> SNATGERFHPLLGRRVLDPAPGARCFTGTVSSDRPAYLGEHWVYDAIVVLGVTYLEMALAAASRLLPGNAADTLIVEDVTVWSPLVLRAGAPARLRLRSEDERFEIHSAEPERSDDESAWTRHATGRIARRQLSPDATGQLPRLDG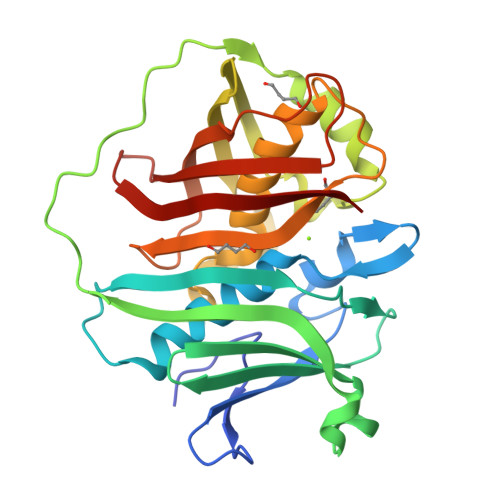EAVELDAYYERMRIYYGPRLRNIRHLERRGREAIGHVCLQGEEAQESASYELHPALLDACFQCVFALIYAHESHREPFVPLGCARIELRARGVREVRVHLRLHPPRSTDHNQTHTADLRLFDMEGRLVASVDALQLKRA To validate some of these predictions experimentally, we applied them to a protein from C. thermophilum, which is homologous to yeast pre-ribosomal export factor Arx1 (Associated with Ribosomal eXport complex). C. thermophilum Arx1 (ctArx1) is thermostable (soluble) up to 53°C at a concentration of 8 mg/ml, whereas the Arx1 from the mesophilic C. globosum (cgArx1) precipitates already at 35°C, corresponding to the OGTs of both organisms. To reveal mechanistic roles for adaptive residues, we determined the 3D structure of ctArx1 that shares the pita-bread fold with methionine-aminopeptidases and Ebp1. By determining the three-dimensional structure of an exemplar protein from C. thermophilum (Arx1), we could also characterise the molecular consequences of some of these mutations.

Expression, purification, crystallization and x-ray structure determination of this protein was successful, supporting the value of C. thermophilum as a model system for structural studies. The two selected adaptive proline mutations (P41, P104) indeed occur in loops of ctArx1 preventing unfolding. Another fundamental concept in thermo-adaptation of proteins is an increased bulkiness of hydrophobic amino acids within the protein core. Direct sequence comparison of ctArx1 with cgArx1 indeed shows that 80% (16/20) of the hydrophobic amino acid exchanges lead to increased bulkiness. Several of these adaptive bulky hydrophobic residues in ctArx1 (F146, F362 and W357) together with V128 form an extended hydrophobic cluster, which together with adaptive C335 leads to a tight packing of helices α3 and α9 to the central beta-sheet. Acquired electrostatic interactions are found between the imino-group of W357 and D124 (β4) linking β4 to α3 more tightly and between adaptive R350 in β13 and E154 stabilizing β13 with respect to helix α3. Mutation of F146, W357 and R350 reduces the thermostability of ctArx1 by about 2°C to 51°C. In addition, mutation of the two hydrophobic residues (F146, W357) on top of the five adaptive mutations leads to a further decrease of ctArx1 thermostability to 47°C. Taken together, these examples of adaptive mutations in the context of the 3D structure of ctArx1 illustrate how individual residues and their interactions contribute to a thermophilic adaptation. By solving the 3D structure of a single thermophilic protein (Arx1 of Cth), we could identify three different types of adaptive mutations : (i) loop rigidity by increased proline frequency, (ii) increased protein core hydrophobicity, and (iii) increased electrostatic interactions stabilizing neighboring secondary structure elements.

>MGHHHHHHMATEKKEADNVAISVDVLTKYKTAAQISEKVLAEVSKLCVPGAKIIDICEQGDKLMEEELSKVYRDKKTNKGFSHPTTVSPAAFITPYTPLRSDEKEAATEIQPGEPIKIQLGAQIDGYGTIVCDTIVAKNANDPDVIEGRQADLFLATYYANEVLLRLMVPPGLLATGTDEEKAKAAAVKPPSQAKISSLLEKVAKAYDCNIIESTTSWLFDKNEIEGKKKIILSPGENIKGEGVPEVGDVWGVEVGCSLGSGKVKQFEQRATLHRRTNNTYALKRPTSRKIYSEVQKKFGTFPFSLRQLEDERDAKSGVIECVRGGVFRQYEVTGDKDNAPVCRLLTTIAITKNGITRIGGPPAWDLSKFKTDKKIEDEEILKILEQPLSKNAGKNKNKKKKKKAKKAAAKPDEGEEESSDEE[4x]>MRGSHHHHHHGSMSELITENMHMKLYMEGTVNNHHFKCTSEGEGKPYEGTQTMRIKVVEGGPLPFAFDILATSFMYGSKTFINHTQGIPDFFKQSFPEGFTWERVTTYEDGGVLTATQDTSLQDGCLIYNVKIRGVNFPSNGPVMQKKTLGWEASTEMLYPADGGLEGRSDMALKLV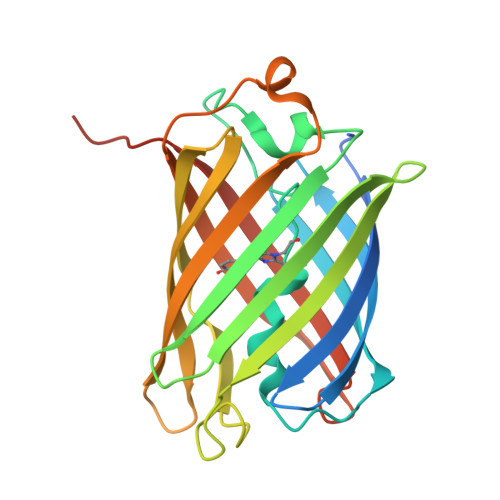GGGHLICNLKTTYRSKKPAKNLKMPGVYYVDRRLERIKEADKETYVEQHEVAVARYCDLPSKLGHKLN[8x]>[4x]GGGRMATTTAGLTDLKFRVVREDFADAVAWVARSLPTRPTIPVLAGVLLTGTDEGLTISGFDYEVSAEVKVSAEIASAGSV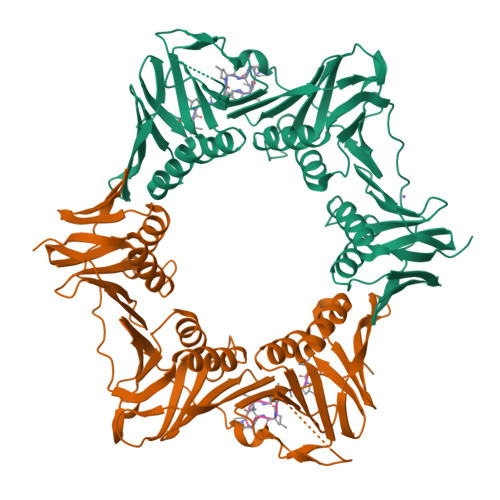LVSGRLLSDITKALPAKPVEVSVEGTRVSLTCGSARFSLPTLAVEDYPALPALPEETGVIASDLFAEAIGQVAVAAGRDDTLPMLTGIRVEISGESVVLAATDRFRLAVRELTWVTTAGDVEAAVLVPAKTLAEAAKAGTDGNQVHLALGSGASVGKDGLLGIRSEGKRSTTRLLDAEFPKFRQLLPAEHTAVATIGVAELTEAIKRVALVADRGAQIRMEFSDDTLKLSAGADDVGRAEEDLPVDFAGEPLTIAFNPTYLTDGLGSLHSERVTFGFTTPSRPAVLRPAGEDDGANGGSGPFPAAKTDYVYLLMPVRLPG;>[4x]XVPTLPLVPXG>MSDTPYKADLSRVHWAGSNSDVDIHLEIFEGDVDSGFMYNSFFRGNSSYVSVQDQSNQARIDRMNTVTIKGRTPGQKLDRESVKNDKLVITVDTVTYASTVMDWQDDWTSPDRWAEIGAQHGYQHARLFDTAHLIQIIKARKWIAPADLKPAFFDGKEYTAAYNADRELFAANIIDAHRQGIEEMVRRDLGGSLTEFITVVSPYVFGLLLDSKKLVNVDYSAGNGNFAERRVGMVNGVRIVESARFPAAAGTSPLGAAFTVDA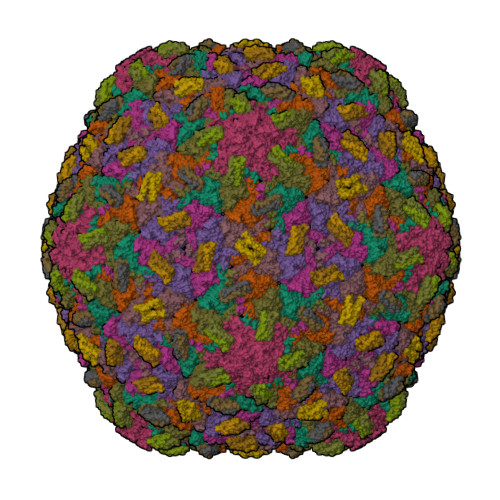DDVACQMVVYHPKMTLVTVEAKPLATNKYPDNPNFSDILDSFTLYTVGQRRPDTSFAVKLTNLP[7x];>MAITTGTTEAQALNMTMRDAVLKVAPGVQQLVQNSSQLTAAEIAIIQTNITALKAAFTAAGA[5x];>[2x]MSLVTATAAQRIALRNTATNLSEQTQVYAQSATAPTAAEAAIVQPYIDAAQAAITAVGAGGATVANGATVAVVNSASADSHNATATVTGTTLTNVKLAATVAFVDNADTITVQNSAGTAVAGTHTATVAAGVISNVKLAATIAPVASGLALTGVTPTGTYTNTVTFTVAAGVITAIVLS> APCPHTYKPVCG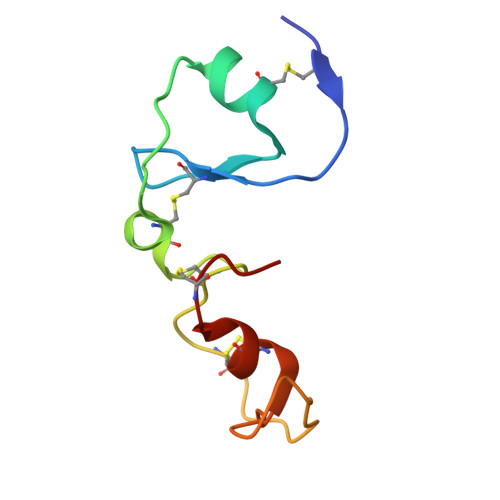ANGEVYDNECFLNKAGIEPAESWETCRGHELCPSVCTEEYDPVCVEGKIYGNRCMQSHFCGKV>[2x]MSIIAINENGFLDKIKGRNPLFTCVISSIETTLSIPISGVHRDVIKYTPSADVELVFYGKSLTLKTPPIDATGSPTPATITRACVELKNIKNLHIDAGAFVKPKIPFIEIDEKPTGRIEEGKAMNNSKELYMKGYLLGKNLDAELLIVGESVPGGTTTALGVLLGLGYDAEGKVSSGSINNPHELKIKVVREGLKKAGINEKSSVFDVLNAVGDKMMPVVAGLAISFAERNKPVILAGGTQMSAVLAVIKEINKKVLDKNLIAIGTTEFVLNDKKGDLKGIVEQIGNVPVLASKFYFEKAKIEGLKNYCKGSVKEGVGAGGIAVYSIVNDLEPTKIREFIENKFYEWYKE

Cobamides (Cbas) are coenzymes used by cells across all domains of life, but de novo synthesis is only found in some bacteria and archaea. Base activation is catalyzed by a phosphoribosyltransferase (PRTase). To gain insights into the mechanism of base activation by the PRTase from Methanocaldococcus jannaschii (MjCobT), we solved crystal structures of the enzyme in complex with substrate and products. The protein fold consists of an eight-stranded mostly parallel β-sheet with connecting α-helices on both sides where the substrate binding pocket is built from the connecting loops and resides at the end of the C-terminal end of β-strands.

The structure of the complex with α-AMP was determined to 1.4 Å resolution. This structure was determined to understand the broad specificity of MjCobT 11. The reaction product was prepared in situ by soaking the crystals in NaMN and adenine. The overall position of the adenine α-ribotide is exceedingly similar to that α-RP so that the primary question is how the enzyme can accommodate nitrogenous bases that differ in both the composition of the aromatic ring and its side chain substitutions. Superposition of the two structures demonstrates that this is accomplished in this instance by conformational changes in the polypeptide chain between Ile 69–Thr 74. This section is ordered with α-AMP and disordered with α-RP. A change in the conformation of this loop, when α-RP is bound, is necessary because the two methyl groups in DMB overlap with the ordered loop seen in the complex with α-ribotide. It is conceivable that the disordered section allows for varied substrate specificity which is a hallmark of CobT. An adenine specific interaction arises between the carbonyl oxygen of Gly 177 and the amino group of adenine, but this does not alter the conformation of the active site. Interestingly, there are no polar interactions between the pyrimidine ring nitrogen N1 and N3 of the purine, which instead lie at van der Waals distance from the surrounding components of the binding pocket.> MRITTKVGDKGSTRLFGGEEVWKDDPIIEANGTLDELTSFIGEAKHYVDEEMKGILEEIQNDIYKIMGEIGSKGKIEGIS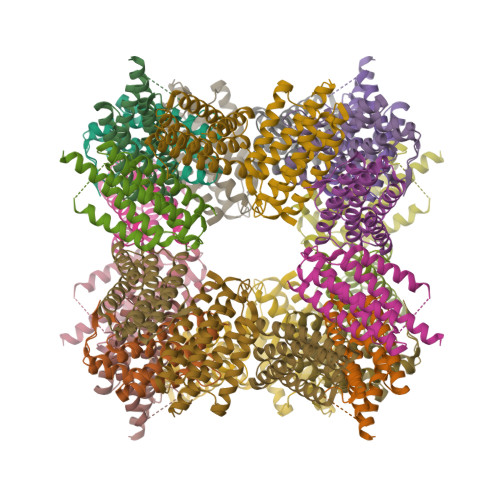EERIKWLAGLIERYSEMVNKLSFVLPGGTLESAKLDVCRTIARRAERKVATVLREFGIGTLAAIYLALLSRLLFLLARVIEIEKNKLKEVRS;> MFTRRGDQGETDLANRARVGKDSPVVEVQGTIDELNSFIGYALVLSRWDDIRNDLFRIQNDLFVLGEDVSTGGKGRTVTMDMIIYLIKRSVEMKAEIGKIELFVVPGGSVESASLHMARAVSRRLERRIKAASELTEINANVLLYANMLSNILFMHALISNKRLNIPEKIWSIHRVSLEHHHHHH HILDH belongs to the short-chain dehydrogenase/reductase (SDR) superfamily. HILDH reduces the racemic AMKP to (2S,3R,4S)-4-HIL and the other seven stereoisomers of 4-HIL in an NADH-dependent manner, suggesting that HILDH has nearly no stereoselectivity with AMKP. HILDH forms a tetrameric structure, and each subunit consists of seven α-helices, seven β-strands and three 310-helices.

The crystal structure of the HILDH-NADH complex has been determined at 2.20 Å resolution. The subunit structure is divided into two subdomains: the main body and the substrate binding unit. The main body of α/β-folding patterns adopts the Rossmann fold, which is conserved in SDRs. The central β-sheet consists of seven parallel β-strands (β1‒β7) sandwiched between two sets of three parallel α-helices (α1, α2 and α7 on one side and α3, α4 and α6 on the opposite side). The α5 helix and three 310-helices are located on the C-terminal side of the Rossmann fold structure to form the substrate binding unit. Additionally, the electron density map of the nicotinamide ring of NADH is observed clearly in each subunit. No significant structural differences were found between the structures of HILDH-NADH and HILDH-NADH-succinate, with RMSDs of 0.2-0.3 Å for α-carbons.

>MRENKIIMISGANSGIGHACIKYFLEKSFHVIALDINNNNLIDYMKTDMPLKVVQIDLSNSEAIHNLFTQLDLEKLSPDILINAAGIREITPVLHLSDDMFKKVIDVNLVAPFILSREVAKRWCESKIKGCIVNIASVSGLMAEPERAAYVASKHALIGLTKQMAMEFGKQNIRVNSISPGVIRTELTEEYFSNKALMSMIKSNQSLDTWGLPQDIVSCIEYLISDQARFITGSNFVIDGGWTAGKNLLEKGELNSKLEGKPIPNPLLGLDSTRTGHHHHHH[4x]1-isothiocyanato-3-methylsulfinyl-propane 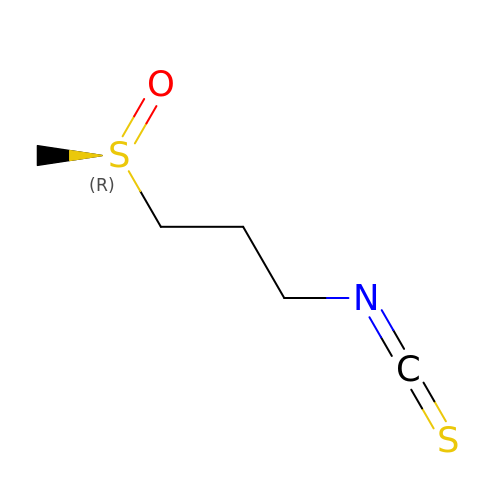| C5 H9 N O S2 | LELAOEBVZLPXAZ-SECBINFHSA-N N-{3-[(3-methylbut-2-en-1-yl){methyl[trans-4-(pyridin-4-yl)cyclohexyl]carbamoyl}amino]phenyl}benzamide 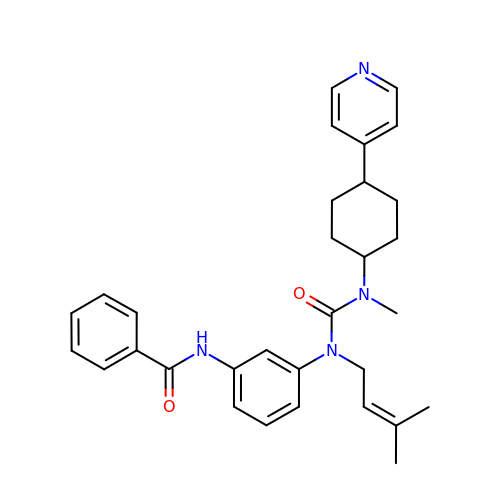| C31 H36 N4 O2 | PITIPWBKTYAGSP-XBTDCMMSSA-N(4aS,6S)-2-amino-6-{(E)-[(4-methylphenyl)imino]methyl}-4-oxo-4,6,7,8-tetrahydropteridine-5(4aH)-carbaldehyde 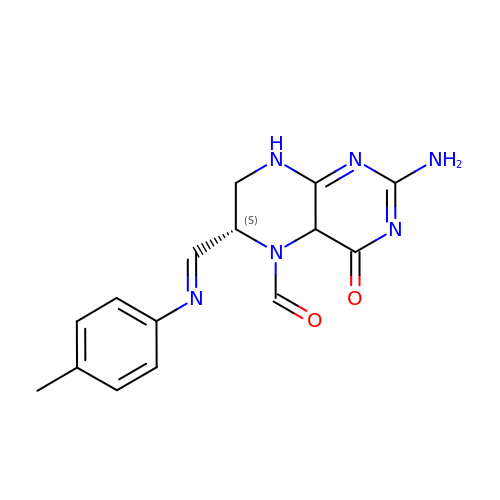| C15 H16 N6 O2 | UDYJDSNAUDQZNM-RMTXVELISA-N>SMGPGVWDPNWDRREPLSLINVRKRNVESGEEELASKLDHYKAKATRHIFLIRHSQYHVDGSLEKDRTLTPLGREQAELTGLRLASLGLKFNKIVHSSMTRAIETTDIISRHLPGVCKVSTDLLREGAPIEPDPPVSHWKPEAVQYYEDGARIEAAFRNYIHRADARQEEDSYEIFICHANVIRYIVCRALQFPPEGWLRLSLNNGSITHLVIRPNGRVALRTLGDTGFMPPDKITRS[3x]

PGAM5 is a mitochondrial membrane protein that functions as an atypical Ser/Thr phosphatase and is a regulator of oxidative stress response, necroptosis, and autophagy. Phosphoglycerate mutase family member 5 (PGAM5) is a mitochondrial membrane protein that belongs to the phosphoglycerate mutase (PGAM) branch of the histidine acid phosphatase superfamily, known also as two-histidine phosphatase (2H-phosphatase). Despite harboring a canonical RHGE catalytic motif, PGAM5 lacks a typical phosphotransferase and/or phosphohydrolase activity for small metabolites, and displays instead a phosphatase function specific for Ser/Thr and, potentially, histidine residues (Takeda et al., 2009, Panda et al., 2016). Overall, the catalytic domain of PGAM5 adopted a classical phosphoglycerate mutase-like fold with the canonical three-layer sandwich topology, which featured a six-stranded β sheet flanked on both sides by α helices with the first four parallel strands arranged in an alternated β/α manner.

To provide structural insights into the role of the N terminus, we next determined the structure of the longer ΔN54-PGAM5 in complex with a phosphate ion. In all three molecules in the asymmetric unit, although most parts of the N-terminal extension to the catalytic domain (amino acids 67–90) was disordered, clear electron density allowed a confident assignment of the WDPNWD motif within the N-terminal region, which packed along the surface of the catalytic core. The accommodation of the WDPNWD motif required both intra- and interdimeric contacts where the tryptophan residues of this motif were accommodated in two hydrophobic grooves, located at intermolecular interfaces created by two different PGAM5 subunits. The presence of the WDPNWD motif triggered a simultaneous occurrence of two interesting structural features that were not observed in the short ΔN90-PGAM5 structures, including the now ordered proline-rich β3-α3 loop and the newly formed interdimeric interactions resulting in a dodecameric assembly. Within the asymmetric unit, one subunit of the dimer associated with the subunit of an adjacent dimer with their α3 helices paired in a reverse manner at the dimer-dimer interface. The WDPNWD-containing N terminus was then positioned in proximity to the proline-rich β3-α3 catalytic loop, leading to an alternated arrangement that resulted in the β3-α3 catalytic loop of one molecule being sandwiched between two neighboring N termini, one from the subunit within the dimer and the other from the protomer of the adjacent dimer. This configuration promoted most likely an ordering of the loop that in turn completed the active site architecture, a feature not observed in the ΔN90-PGAM5 structure. Based on the dimer-dimer arrangement, an application of the crystallographic symmetry led to a single-layer, doughnut-like dodecameric assembly with an outer dimension of 138 × 48 Å and a radius of 65 Å for the inner hole.> SGGNAEEITEKATLVGIEAWLLAKDEEQKKKVRTLNRQVKKLLQQNDL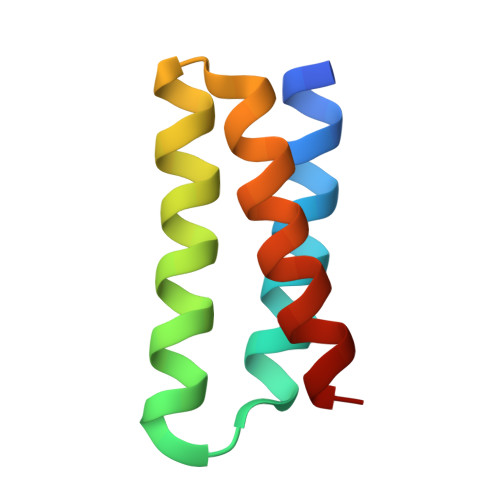DQAKRVLDQLKSVLEDLKS> SNHLVKGRSVYELDCIPLWGTVSIQGNRSEMEDAFAVSPHFLKLPIKMLMGDHEGMSPSLTHLTGHFFGVYDGHGGHKVADYCRDRLHFALAEEIERIKDELSKR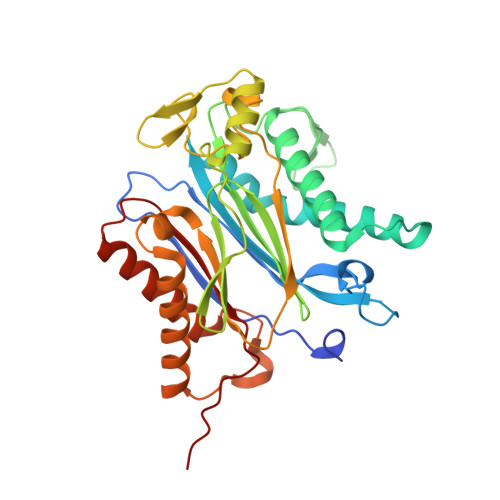NTGEGRQVQWDKVFTSCFLTVDGEIEGKIGRAVVGSSDKVLEAVASETVGSTAVVALVCSSHIVVSNCGDSRAVLFRGKEAMPLSVDHKPDREDEYARIENAGGKVIQWQGARVFGVLAMSRSIGDRYLKPYVIPEPEVTFMPRSREDECLILASDGLWDVMNNQEVCEIARRRILMWHKKNGAPPLAERGKGIDPACQAAADYLSMLALQKGSKDNISIIVIDLKAQRKFKTRT> MTVDFLSMVKYTPLFISGLIMTLKLTFLAVTIGVLMGLFIALMKMSSIKPIKLVASSYIEVIRGTPLLVQLLLIYNGLMQFGMN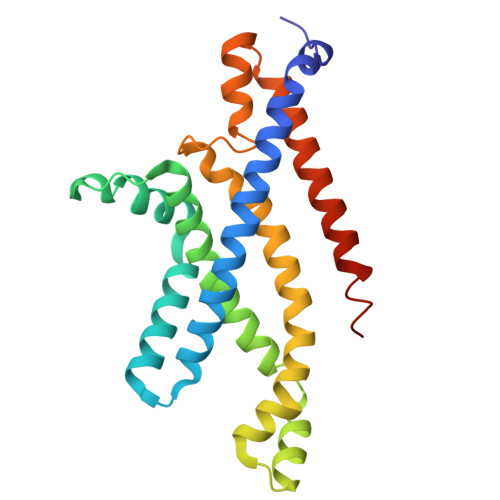IPAFTAGVSALAINSSAYVAEIIRAGIQAVDPGQNEAARSLGMTHAMAMRYVIIPQAIKNILPALGNEFIVMLKESAIVSVIGFADLTRQADIIQSVTYRYFEPYIIIAAIYFVMTLTFSKLLSLFERRLRAGDIR> MIFEVLKILTDEVNQNFKGLEMEDSEVVLNNVALIDSQQDVATELQNKVILSMINLREEVTMKNFPNNVLEGTKVTYKNPKLNINLFLIFCANRTGYKKSLSDLSRILEFFQHKSVFTQSNTSFDRDLEEMENVKNFRFTMELFTPTFEELNYIWGTLGGRQYPSVFYKL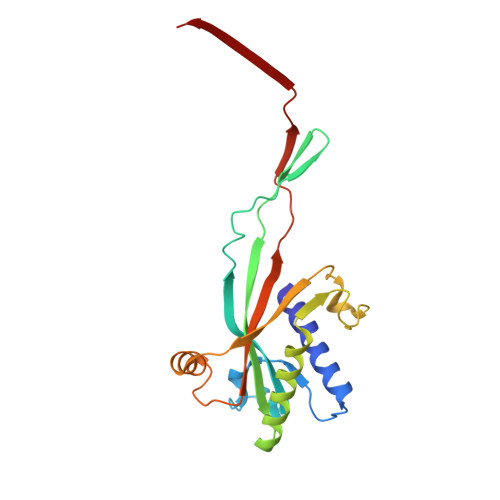NLIVIDRDATTSEEGVITNIHRNYETL> NGEPDIAQLKGLSPSQRQAYAVQLKNRGNHFFTAKNFNEAIKYYQYAIELDPNEPVFYSNISACYISTGDLEKVIEFTTKALEIKPDHSKALLRRASANESLGNFTDAMFDLSVLSLNGDFDGASIEPMLERNLNKQAMKVLNENLSKDEGRGSQVLPSNTSLASFFGIFDSHLEVSSVNTSSNYDTAYALLSDALQRLYSATDEGYLVANDLLTKSTDMYHSLLSANTVDDPLRENAALALCYTGIFHFLKNNLLDAQVLLQESINLHPTPNSYIFLALTLADKEN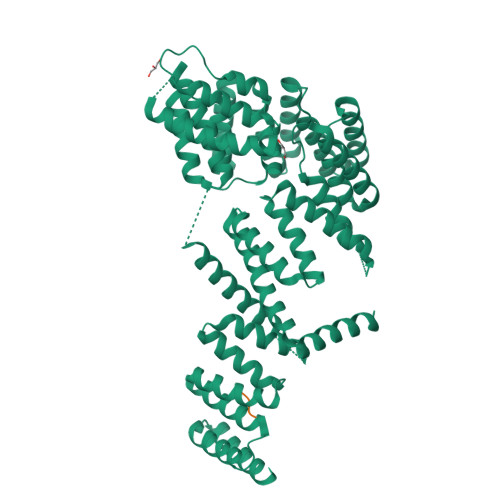SQEFFKFFQKAVDLNPEYPPTYYHRGQMYFILQDYKNAKEDFQKAQSLNPENVYPYIQLACLLYKQGKFTESEAFFNETKLKFPTLPEVPTFFAEILTDRGDFDTAIKQYDIAKRLEEVQEKIHVGIGPLIGKATILARQSSQDPTQLDEEKFNAAIKLLTKACELDPRSEQAKIGLAQLKLQMEKIDEAIELFEDSAILARTMDEKLQATTFAEAAKIQKRLRADPIISAKMELTLARYRAKGML;> PEAEGPTVEEVD> MNLKDSIGLRIKTERERQQMSREVLCLDGAELTVRQLIRIEKGESLPSLDRLSYIAKRLGKSMTELLDQDNITIPDEYYEMKNRLIKFPTYRNPDRIKSKLTLIEEVYEKFFDILPEEELLTLDILENILSFTSWEESPKVEEIYEDLFEQVKRKRKFSTNDLLVIDYYFFHLYGRKQYDKKLFERIIKRVLNQEIWTDDVYNIVLFNDLMA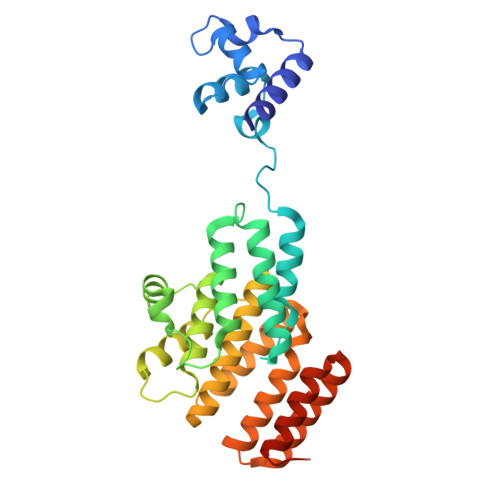IAALKIFHNSFSDFLTVVDKALAVIEKSQLYSYKPSVFVLKAKYELLHKENKKEAAENYDKAIVFASVLEDSVLEESIKAGKLADGLGAGWSHPQFEK> GSVLDGPYQPTTFKPPNDYWLLISSNTDGVVYESTNNSDFWTAVIAVEPHVSQTNRQYVLFGENKQFNVENNSDKWKFFEMFKGSGQSDFSNRRTLTSNNRLVGMLKYGGRVWTFHGETPRATTDSSNTADLNNISIIIHSEFYIIP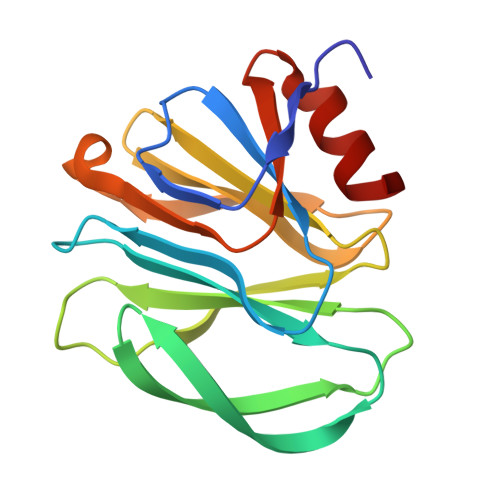RSQESKCNEYINNGL>[4x]MAAACRSVKGLVAVITGGASGLGLATAERLVGQGASAVLLDLPNSGGEAQAKKLGNNCVFAPADVTSEKDVQTALALAKGKFGRVDVAVNCAGIAVASKTYNLKKGQTHTLEDFQRVLDVNLMGTFNVIRLVAGEMGQNEPDQGGQRGVIINTASVAAFEGQVGQAAYSASKGGIVGMTLPIARDLAPIGIRVMTIAPGLFGTPLLTSLPEKVCNFLASQVPFPSRLGDPAEYAHLVQAIIENPFLNGEVIRLDGAIRMQP;> SNAFSLKTMSPQNTKATNLIAKARYLRKDEGSNKQVYSVPHFFLAGAAKERSQMNSQTEDHALAPVRNTIQLPTQPLNSEEWDKLKEDLKENTGKTSFESWIISQMAGCHSSIDVAKSLLAWVAAKNNGIVSYDLLVKYLYLCVFHMQTSEVIDVFEIMKARYKTLEPRGYSLLIRGLIHSDRWREALLLLEDIKKVITPSKKNYNDCIQGALLHQDVNTAWNLYQELLGHDIVPMLETLKAFFDFGKDIKDDNYSNKLLDILSYLRNNQLYPGESFAHSIKTWFESVPGKQWKGQFTTVRKSGQCSGCGKTIESIQLSPEEYECLKGKIMRDVIDGGDQYRKTTPQELKRFENFIKSRPPFDVVIDGLNVAKMFPKVRESQLLLNVVSQLAKRNLRLLVLGRKHMLRRSSQWSRDEMEEVQKQASCFFADDISEDDPFLLYATLHSGNHCRFITRDLMRDHKACLPDAKTQRLFFKWQQGHQLAIVNRFPGSKLTFQRILSYDTVVQTTGDSWHIPYDEDLVERCSCEVPTKWLCLHQKT;> SNAMSSKIPAVTYPKNESTPPSEELELDKWKTTMKSSVQEECVSTISSSKDEDPLAATREFIEMWRLLGREVPEHITEEELKTLMECVSNTAKKKYLKYLYTKEKVKKARQIKKEMKAAAREEAKNIKLLETTEEDKQKNFLFLRLWDRNMDIAMGWKGAQAMQFGQPLVFDMAYENYMKRKELQNTVSQLLESEGWNRRNVDPFHIYFCNLKIDGALHRELVKRYQEKWDKLLLTSTEKSHVDLFPKDSIIYLTADSPNVMTTFRHDKVYVIGSFVDKSMQPGTSLAKAKRLNLATECLPLDKYLQWEIGNKNLTLDQMIRILLCLKNNGNWQEALQFVPKRKHTGFLEISQHSQEFINRLKKAKT

Human mitochondrial transcripts contain messenger and ribosomal RNAs flanked by transfer RNAs (tRNAs), which are excised by mitochondrial RNase (mtRNase) P and Z to liberate all RNA species. Mammalian mitochondrial RNase P is evolutionarily unique because it is a multisubunit protein complex consisting of PRORP (also known as MRPP3), which is homologous to single-subunit PRORPs, and the two additional subunits TRMT10C (also known as MRPP1) and SDR5C1 (also known as MRPP2). This multimeric complex carries out both pre-tRNA cleavage and methylation, and is thus a central player in mitochondrial gene expression. In contrast to nuclear or bacterial RNase P, mtRNase P is not a ribozyme but comprises three protein subunits that carry out RNA cleavage and methylation by unknown mechanisms.

To investigate the mechanism of mitochondrial pre-tRNA processing and methylation, we reconstituted human mtRNase P and determined its structure using single-particle cryo-EM at an overall resolution of 3.0 Å. The structure contains TRMT10C, four copies of SDR5C1, and PRORP in its active conformation. The substrate pre-tRNA is tightly bound, with the methyl-acceptor base 9 flipped into the TRMT10C methyltransferase domain and the 5′ end positioned in the PRORP active site for cleavage. Human mtRNase P adopts an elongated structure around the centrally embedded pre-tRNA. SDR5C1 forms a rectangular, symmetric tetramer, as previously reported. Its dehydrogenase active sites are near the binding interface with TRMT10C, and each SDR5C1 monomer has a NADH cofactor bound in its dehydrogenase active site. The C-terminal methyltransferase domain of TRMT10C binds on top of the SDR5C1 tetramer, with its active site facing sideways. It is anchored to the SDR5C1 tetramer by the adapter helix (TRMT10C α4, residues 183–202), which precedes the methyltransferase domain and was not included in the previous crystal structure. R181 protrudes into the anticodon loop and interacts with the C2 carbonyl of U33. This interaction is specific to pyrimidine nucleobases and is likely crucial for correct substrate recognition, as this position is conserved as U or C in tRNAs, and mutations of R181 cause mitochondrial RNA processing defects and respiratory chain deficiency in patients. The methyltransferase active site is positioned directly adjacent to the junction between the acceptor arm and the D arm, where G9 is flipped out of the tRNA fold and buried into the active site, stacking against the conserved residue V313. In the mtRNase P complex, PRORP adopts a more ‘open’ conformation with respect to the angle between its nuclease and PPR domains.2-methyl-~{N}-(2-methylpropyl)imidazo[1,2-a]pyridine-3-carboxamide 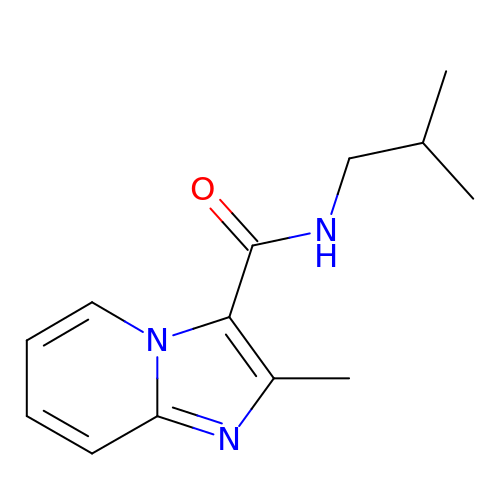| C13 H17 N3 O | QQNPIZGIGPGFPW-UHFFFAOYSA-N> PISPIETVPVKLKPGMDGPKVKQWPLTEEKIKALVEICTEMEKEGKISKIGPENPYNTPVFAIKKKDSTKWRKLVDFRELNKRTQDFWEVQLGIPHPAGLKKKKSVTVLDVGDAYFSVPLDEDFRKYTAFTIPSINNETPGIRYQYNVLPQGWKGSPAIFQSSMTKILEPFKKQNPDIVIYQYMDDLYVGSDLEIGQHRTKIEELRQHLLRWGLTTPDKKHQKEPPFLWMGYELHPDKWTVQPIVLPEKDSWTVNDIQKLVGKLNWASQIYPGIKVRQLCKLLRGTKALTEVIPLTEEAELELAENREILKEPVHGVYYDPSKDLIAEIQKQGQGQWTYQIYQEPFKNLKTGKYARMRGAHTNDVKQLTEAVQKITTESIVIWGKTPKFKLPIQKETWETWWTEYWQATWIPEWE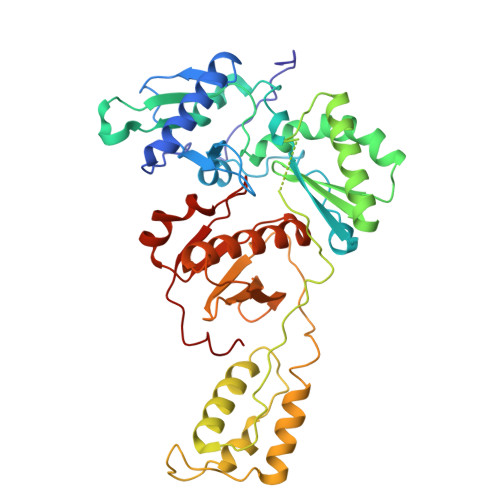FVNTPPLVKLWY>[3x]GSHMAETAELNLPGGQSISLPIFEGTEQEKAFDIGKLRDATGYVTLDSGYKNTGACKSAITFLDGEEGILRYRGYPIEQLAENSSFLEVAYLLIYGHLPTEAELKDFSGHITKHTLVHEDIRKIFDGFPSSTHPMAILSSLTCALTGFYPESISPNQTPEAIDLTIVRLMAKMSTIAAWTYKNSVGHPLNYPRNDLDYCANFLYMMFSFPTEKYEINPVIVSALNKLLILHADHEQNCSTST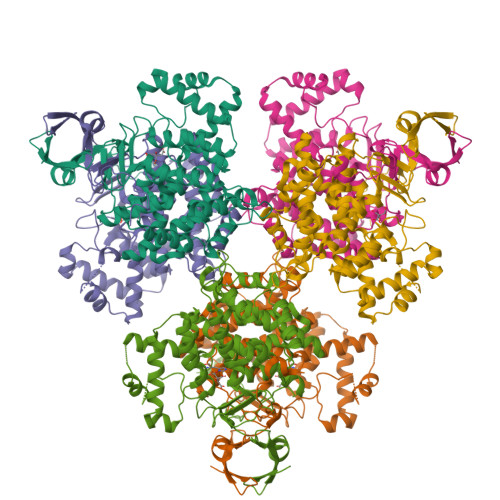VRLVGSANASLYGSVSAGINALWGPLHGGANQEVIEMLEAIEKDGGDTSKFIAQAKDKNSGFRLMGFGHRVYKNFDPRAKIIKVAADEVLQALGMQNSPLLKIATELEQAALTDQYFIDRKLYPNVDFYSGIIYKALGIPTEMFTVMFALGRLPGWIAQWKEMRENKEPIGRPRQIYVGETERNYVPMTERK>[3x]MGSTKPRFTTGLVYDTLMLKHQCTCGSSSSHPEHAGRIQSIWSRLQETGLRGKCECIRGRKATLEELQTVHSEAHTLLYGTNPLNRQKLDSKKLLGSLASVFVRLPCGGVGVDSDTIWNEVHSAGAARLAVGCVVELVFKVATGELKNGFAVVRPPGH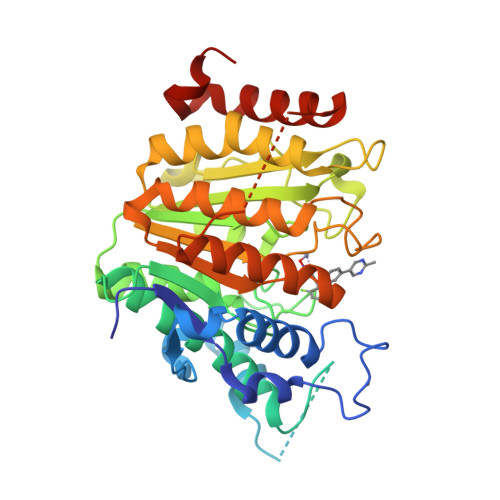HAEESTPMGFCYFNSVAVAAKLLQQRLSVSKILIVDWDVHHGNGTQQAFYSDPSVLYMSLHRYDDGNFFPGSGAPDEVGTGPGVGFNVNMAFTGGLDPPMGDAEYLAAFRTVVMPIASEFAPDVVLVSSGFDAVEGHPTPLGGYNLSARCFGYLTKQLMGLAGGRIVLALEGGHDLTAICDASEACVSALLGNELDPLPEKVLQQRPNANAVRSMEKVMEIHSKYWRCLQRHHHHHH> GSHSWRHIRAEGLDSSYTVLFGKAEADEIFQELEKEVEYFTGALARVQVFGKWHSVPRKQATYGDAGLTYTFSGLTLSPKPWIPVLERIRDHVSGVTGQTFNFVLINRYKDGSDHIGEHRDDCRELAPGSPIASVSFGASRDFVFRHKDSRGKSPSRRVAVVRLPLAHGSLLMMNHPTNTHWYHSLP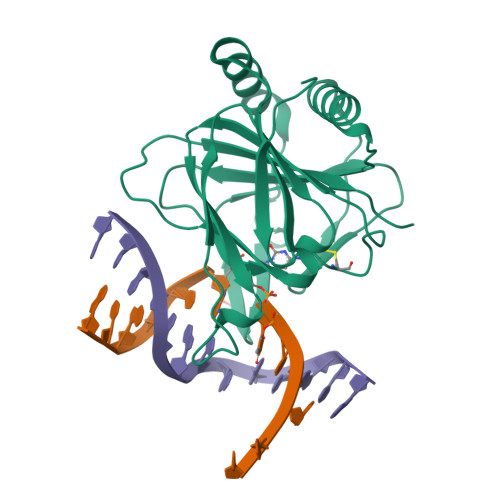VRKKVLAPRVNLTFRKILLTKK For example, unfractionated saliva from Rhipicephalus sanguineus inhibits dendritic cell maturation and differentiation; Salp15, an Ixodes scapularis salivary gland protein, inhibits dendritic cell secretion of pro-inflammatory cytokines; while Japanin, an 18 kDa protein recently isolated from the salivary glands of a hard tick, Rhipicephalus appendiculatus (the Brown Ear Tick), works through currently undefined mechanisms to block DC differentiation from monocytes and inhibits upregulation of co-stimulatory molecules and pro-inflammatory cytokines in response to stimuli. Japanin is predicted from sequence data to be a lipocalin, a member of a family of ubiquitous small proteins found in both prokaryotes and eukaryotes. To provide insight into Japanin’s mechanism of action, we here present two crystal structures of the protein. They reveal that Japanin exists in complex with cholesterol and that it forms a dimer, as well as confirming the prediction from primary sequence that it adopts the lipocalin fold. As was predicted from the sequence, the protein folds as a lipocalin, with an 8-stranded anti-parallel barrel at its centre.

We obtained two crystal structures of recombinantly expressed R. appendiculatus Japanin: (i) a tetragonal form with one copy per asymmetric unit (data to 2.2 Å) and (ii) an orthorhombic one with two molecules per asymmetric unit (data to 2.4 Å), both in complex with cholesterol. In the tetragonal crystals, the same dimer is formed by the asymmetric unit and a symmetry-related molecule across a twofold axis. The tetragonal crystal-form dimer and the orthorhombic crystal-form dimer superpose with an rmsd of 1.5 Å over 297 Cαs. All three crystallographically-independent molecules show the same overall structure, and each molecule in the crystals binds one molecule of cholesterol. The three crystallographically-independent molecules superimpose with an overall Cα rmsd of 1.3 Å across 152 residues (overlap computed with the program Theseus10). The main sites of conformational mobility are the hairpin loop 48–58, the loop 105–112 and the C-terminus, residues 145–152. Two disulphide bonds are observed (Japanin residues Cys28-Cys150 and Cys114-Cys138), the latter taking two alternative conformations. In the Japanin crystals, the cholesterol ligand is completely sequestered inside the protein, except for the –OH group at position 3, which points towards a solvent accessible cavity.

> TPSMPAINTQTLYLAGHSSKLFERNVGCVKTRYLNQTGDWVTRSLIYVFTFDTEPWVTQAGAFQVKWEPYSPLLRVKASDYVRDNLGAKPDYFIRTYDNDFLLLSDLKEVRSTCSLWVTLKYVDRIPETINRTFYTICPDPVPVPFDERCYPGGHHHHHH> GDPVEDIIHDALGNTARRAISGATNVESAADTTPSSHRLETGRVPALQAAETGATSNATDENMIETRCVINRNGVLETTINHFFSRSGLVGVVNL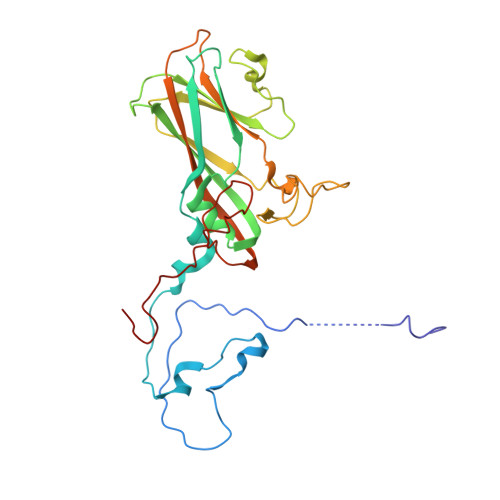TDGGDTTGYATWDIDIMGFVQLRRKCEMFTYMRFNAEFTFVTTTKSGEARPYMLQYMYVPPGAPKPTGRDAFQWQTATNPSVFVKLTDPPAQVSVPFMSPASAYQWFYDGYPTFGQHPETSNTTYGLCPNNMMGTFAVRVVSREASQLKLQTRVYMKLKHVRAWVPRPIRSQPYLLKNFPNYDSSKITNSARDRSSIKQANM> CGRVRDFVAKLANNTHQHVFDDLRGSVSLSWVGDSTGVILVLTTFHVPLVIMTFGQSKLYRSEDYGKNFKDITDLINNTFIRTEFGMAIGPENSGKVVLTAEVSGGSRGGRIFRSSDFAKNFVQTDLPFHPLTQMMYSPQNSDYLLALSTENGLWVSKNFGGKWEEIHKAVCLAKWGSDNTIFFTTYANGSCKADLGALELWRTSDLGKSFKTIGVKIYSFGLGGRFLFASVMADKDTTRRIHVSTDQGDTWSMAQLPSVGQEQFYSILAANDDMVFMHVDEPGDTGFGTI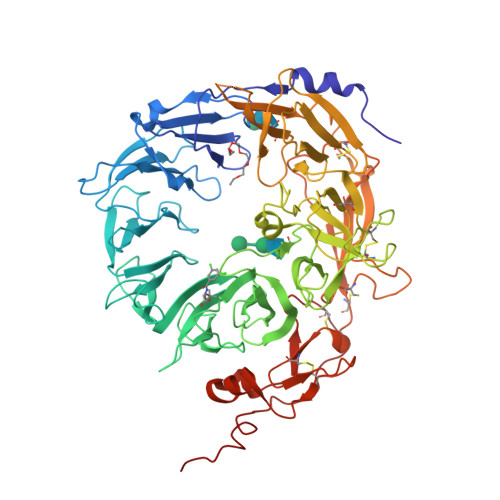FTSDDRGIVYSKSLDRHLYTTTGGETDFTNVTSLRGVYITSVLSEDNSIQTMITFDQGGRWTHLRKPENSECDATAKNKNECSLHIHASYSISQKLNVPMAPLSEPNAVGIVIAHGSVGDAISVMVPDVYISDDGGYSWTKMLEGPHYYTILDSGGIIVAIEHSSRPINVIKFSTDEGQCWQTYTFTRDPIYFTGLASEPGARSMNISIWGFTESFLTSQWVSYTIDFKDILERNCEEKDYTIWLAHSTDPEDYEDGCILGYKEQFLRLRKSSMCQNGRDYVVTKQPSICLCSLEDFLCDFGYYRPENDSKCVEQPELKGHDLEFCLYGREEHLTTNGYRKIPGDKCQGGVNPVREVKDLKKKCTSNFLSPE>GPYASLTEIEHLVQSVCKSYRETCQLRLEDLLRQRSNIFSREEVTGYQRKSMWEMWERCAHHLTEAIQYVVEFAKRLSGFMELCQNDQIVLLKAGAMEVVLVRMCRAYNADNRTVFFEGKYGGMELFRALGCSELISSIFDFSHSLS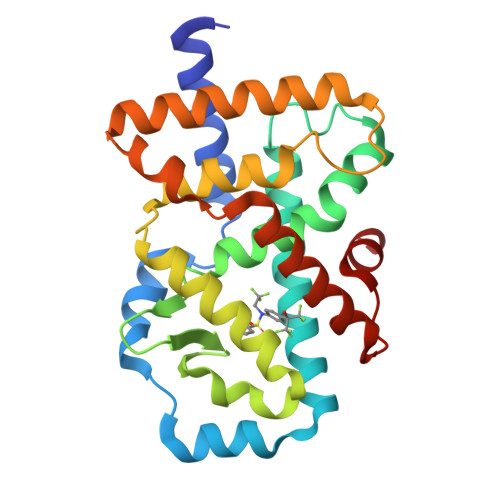ALHFSEDEIALYTALVLINAHRPGLQEKRKVEQLQYNLELAFHHHLSKTHRQSILAKLPPKGKLRSLCSQHVERLQIFQHLHPIVVQAAFP[2x]> TDVATVVSQAKAQMKEAYYTYSHTVTETGQFPDIKDVYAAYNKAKQAYANAVAVVNKAGGAKKDAYLADLQAIYETYVFKANPKSGEARVATYIDAYNYATK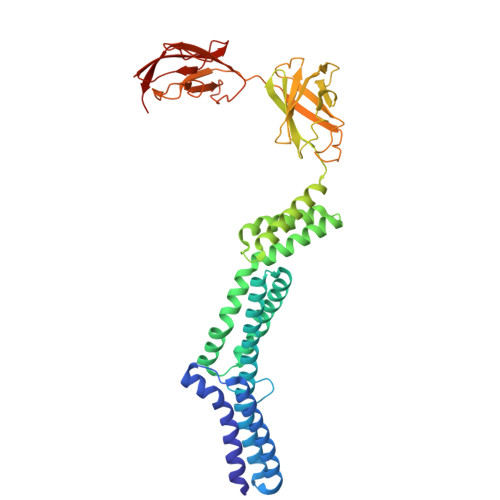LDKMRQELKAAVDAKDLKKAEELYHKISYELKTRTVILDRVYGQSTRELLRSTFKADAQALRDRLIYDITVAMKAREAQDAVKAGNLDKAKAALDQVNQYVSKVTDAFKAELQKAAQDAKAAYEAALTPKVESVSAIDSTSFKVTFTKPVDKATAIPKNFSITLKGTETKLYPKSVEVSESGLTATVTLYDTLVDGKTYTVVTSGLKDTAGKEFETSTNEFTYNKPVPASITFNFNKLPEDSAVDLTKYVTVKDAAGNVIKSGFELEFTSSEKLTQGKFINTTGKKSVIVNATVKGTNVTTGNVILAVED> GAMSETSVNRGPEKIRPECFELLRVLGKGGYGKVFQVRKVTGANTGKIFAMKVLKKAMIVRNAKDTAHTKAERNILEEVKHPFIVDLIYAFQTGGKLYLILEYLSGGELFMQLEREGIFMEDTACFYLAEISMALGHLHQKGIIYRDLKPENIMLNHQGHVKLTDFGLCKESIHDGTVTHTFCGTIEYMAPEILMRSGHNRAVDWWSLGALMYDMLTGAPPFTGENRKKTIDKILKCKLNL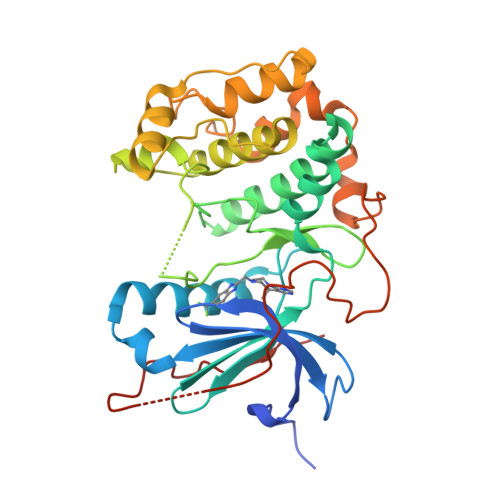PPYLTQEARDLLKKLLKRNAASRLGAGPGDAGEVQAHPFFRHINWEELLARKVEPPFKPLLQSEEDVSQFDSKFTRQTPVDSPDDSTLSESANQVFLGFEYVAPS> GAMASSNSKKELPPAELTDFKEEVVLSKQWSRSVGDGQGDLYNLLEPAVDGSTIYAASAEGRVMAIQRETGDVLWKKDLERPVSGGVGVGYGLVLVGTLRGDVIALDEATGKKKWTKRVNSEVLSAPATNGDVVVVQTQDDKLIGLDAASGDQRWIYESTVPVLTLRGTGAPLIAGNMALAGLASG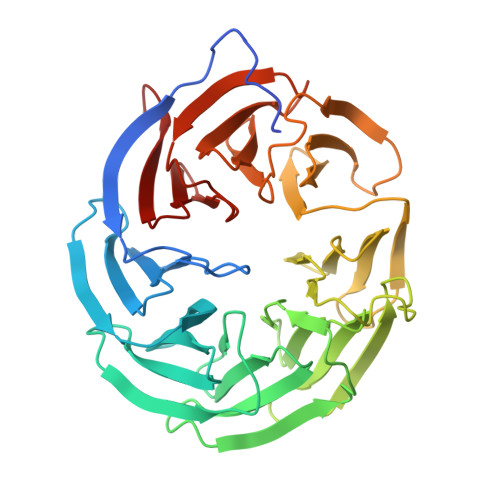KVVAVDVQRGLPIWEQRVAIPQGRSELDRVVDIDGGLLLSGDTLYVVSYQGRAAALDVNSGRLLWQREASSYVGVAEGFGNIYVSQASGSVEGLDSRGASSLWNNDALARRQLSAPAVFSSNVVVGDLEGYVHLLSQVDGRFVGRERVDSDGVRVRPLVVGSWMYVFGNGGKLVAYTIRPG> LPQSVSRAAITAAYRRPETEAVSMLLEQARLPQPVAEQAHKLAYQLADKLRNQKN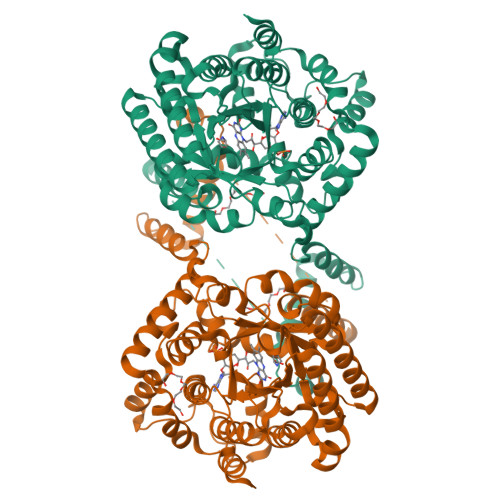ASGRAGMVQGLLQEFSLSSQEGVALMCLAEALLRIPDKATRDALIRDKISNGNWQSHIGRSPSLFVNAATWGLLFTGKLVSTHNEASLSRSLNRIIGKSGEPLIRKGVDMAMRLMGEQFVTGETIAEALANARKLEEKGFRYSYDMLGEAALTAADAQAYMVSYQQAIHAIGKASNGRGIYEGPGISIKLSALHPRYSRAQYDRVMEELYPRLKSLTLLARQYDIGINIDAEESDRLEISLDLLEKLCFEPELAGWNGIGFVIQAYQKRCPLVIDYLIDLATRSRRRLMIRLVKGAYWDSEIKRAQMDGLEGYPVYTRKVYTDVSYLACAKKLLAVPNLIYPQFATHNAHTLAAIYQLAGQNYYPGQYEFQCLHGMGEPLYEQVTGKVADGKLNRPCRISAPVGTHETLLAYLVRRLLENGANTSFVNRIADTSLPLDELVADPVTAVEKLAQQEGQTGLPHPKIPLPRDLYGHGRDNSAGLDLANEHRLHHHHHH{2-[3-(hex-1-yn-1-yl)pyridinium-1-yl]ethane-1,1-diyl}bis(phosphonate) | C13 H16 N O6 P2 | 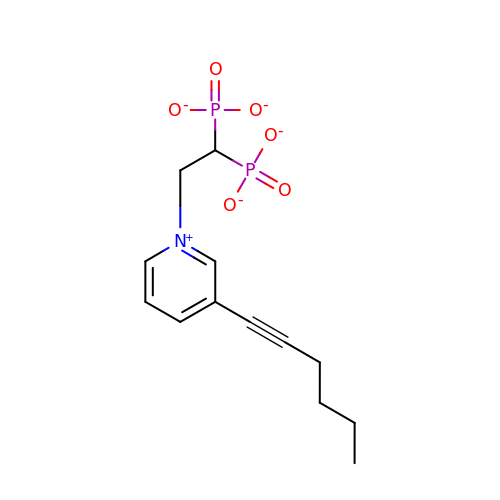SRPWAHINDKLPAE-UHFFFAOYSA-K> MSGAA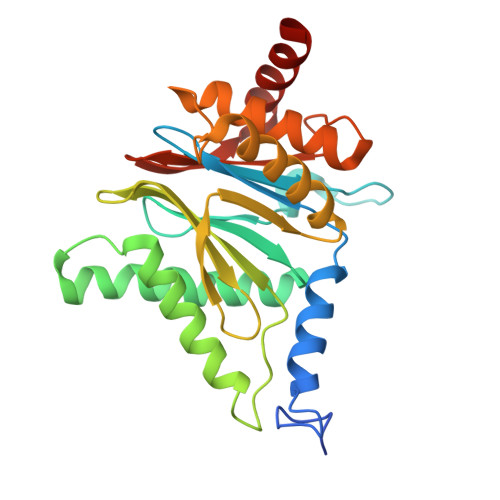AASAAGYDRHITIFSPEGRLYQVEYAFKATNQTNINSLAVRGKDCTVVISQKKVPDKLLDPTTVSYIFCISRTIGMVVNGPIPDARNAALRAKAEAAEFRYKYGYDMPCDVLAKRMANLSQIYTQRAYMRPLGVILTFVSVDEELGPSIYKTDPAGYYVGYKATATGPKQQEITTNLENHFKKSKIDHINEESWEKVVEFAITHMIDALGTEFSKNDLEVGVATKDKFFTLSAENIEERLVAIAEQD>[4x]MVEYHIPSWDEIEDAVFSIGEALVKSNYIPDVLIAVLTGGIIPAKLLSDLLDLKVIRYIDIKFYRSVGKTESKPVIRSVYTDSLEGKKVLVVD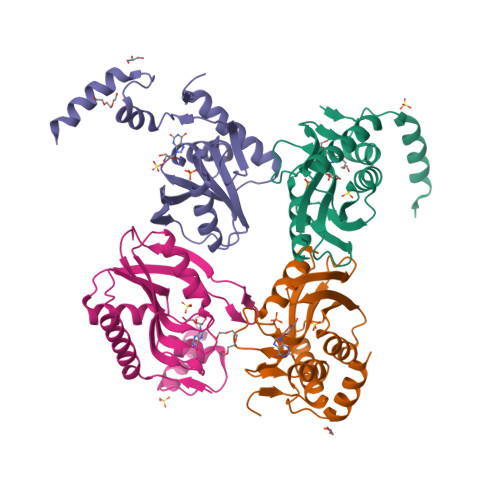DVADTGETLEAVSNVITMFNPAKVMTAALYLKPWSKRIPDFYYKQIDKWIIFPWDKWDVVRENSNVPVDKKERFLNLYNQLLKIRK> MKNTSKFQNVVIVTIVGWLVLFVFLPNLMIIGTSFLTRDDASFVKMVFTLDNYTRLLDPLYFEVLLHSLNMALIATLACLVLGYPFAWFLAKLPHKVRPLLLFLLIVPFWTNSLIRIYGLKIFLSTKGYLNEFLLWLGVIDTPIRIMFTPSAVIIGLVYILLPFMV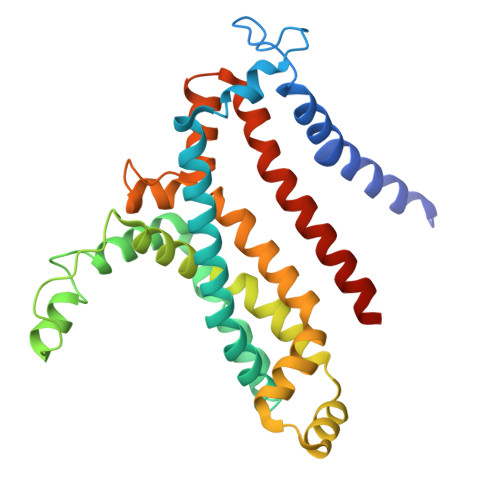MPLYSSIEKLDKPLLEAARDLGASKLQTFIRIIIPLTMPGIIAGCLLVMLPAMGLFYVSDLMGGAKNLLIGNVIKVQFLNIRDWPFGAATSITLTIVMGLMLLVYWRASRLLNKKVELE> TEQATTTDELAFTRPYGEQEKQILTAEAVEFLTELVTHFTPQRNKLLAARIQQQQDIDNGTLPDFISETASIRDADWKIRGIPADLEDRRVEITGPVERKMVINALNANVKVFMADFEDSLAPDWNKVIDGQINLRDAVNGTISYTNEAGKIYQLKPNPAVLICRVRGLHLPEKHVTWRGEAIPGSLFDFALYFFHNYQALLAKGSGPYFYLPKTQSWQEAAWWSEVFSYAEDRFNLPRGTIKATLLIETLPAVFQMDEILHALRDHIVGLNCGRWDYIFSYIKTLKNYPDRVLPDRQAVTMDKPFLNAYSRLLIKTCHKRGAFAMGGMAAFIPSKDEEHNNQVLNKVKADKSLEANNGHDGTWIAHPGLADTAMAVFNDILGSRKNQLEVMREQDAPITA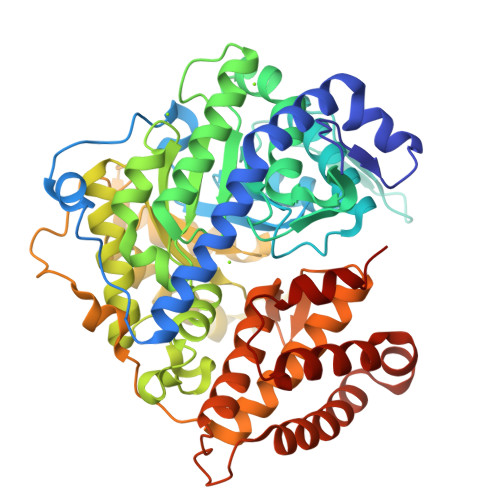DQLLAPCDGERTEEGMRANIRVAVQYIEAWISGNGCVPIYGLMEDAATAEISRTSIWQWIHHQKTLSNGKPVTKALFRQMLGEEMKVIASELGEERFSQGRFDDAARLMEQITTSDELIDFLTLPGYRLLA> PICTTRDGVEIFYKDWGQGRPVVFIHGWPLNGDAWQDQLKAVVDAGYRGIAHDRRGHGHSTPVWDGYDFDTFADDLNDLLTDLDLRDVTLVAHSMGGGELARYVGRHGTGRLRSAVLLSAIPPVMIKSDKNPDGVPDEVFDALKNGVLTERSQFWKDTAEGFFSANRPGNKVTQGNKDAFWYMAMAQTIEGGVRCVDAFGYTDFTEDLKKFDIPTLVVHGDDD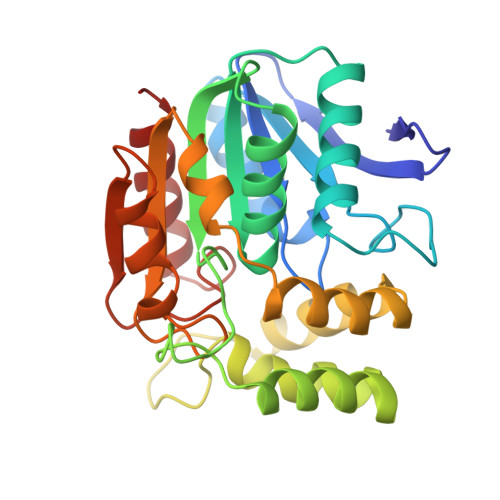QVVPIDATGRKSAQIIPNAELKVYEGSSHGIAMVPGDKEKFNRDLLEFLNK>GPSQNAIKRFMTLFSGREDVFSIQYEGGYRPIRRPLNFQDIKNHFSGKKTLGIYLLKKNDTVKFAAYDIDIKKHYLNREDKFVYEENSKKVAKRLSRELNLENITHYFEFTGNRGYHIWIFFDIPVSAYKIK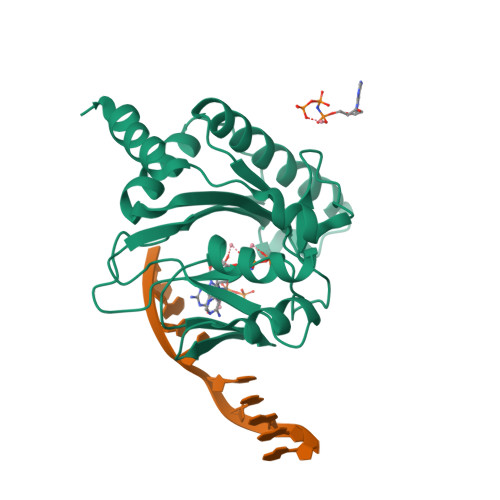YIMEKILDRIELEEGIDVEIFPKQTSLNGGLGNLIKVPLGVHKKTGKKCLFVDNDFNVIENQIEFLNNIKENKATEINKLFREIFNE[3x]>[2x]MGAERDESGAGAAVLVPLLGFG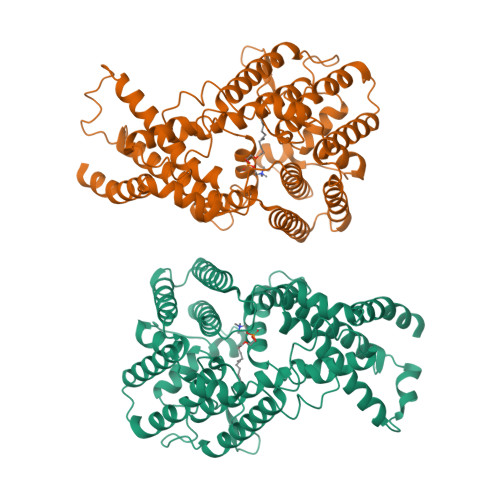SNRPAGPAEKMAVAGSGWSLARVAEALGSSEQALRLIVSILMGYPFALFQRYFLFQKETYLIHLYNVFTGLSIAYFNFGMQFFHSLLCVLIQFLILRLMGRTVTAVFTTFVFQMTYLMAGYYFTATEHYDIKWTMPHCVLTLKLIGLAIDYYDGGKDPELLTPEQRRFAVRGVPTLLEVSGFSYFYGAFMVGPQFSMTDYQKLAKGEMTDVPGQRPNSFVPALKRLSLGLLFLVTYTLSSPYISEEYLISDDYMEKPFWFRCGYILVWGKIILYKYVTCWLVTEGVCILVGLGYNGNDQNGKPVWDACANMKVWLYETTPLFTGTIASFNINTNAWVARYVFKRLKFLGNKLLSQALALFFLAIWHGLHSGYLVCFQMELLIVIVERQVINLVRDSPTLSTLASITALQPIFYVLQQTNHWMFMGYSLVPFCLFTWDKWMKVYKSIYFLGHVLFFTLLLVLPYIRKLLVPRKEKLKKAE>[2x]LECHNQQSSQTPTTTGCSGGETNCYKKRWRD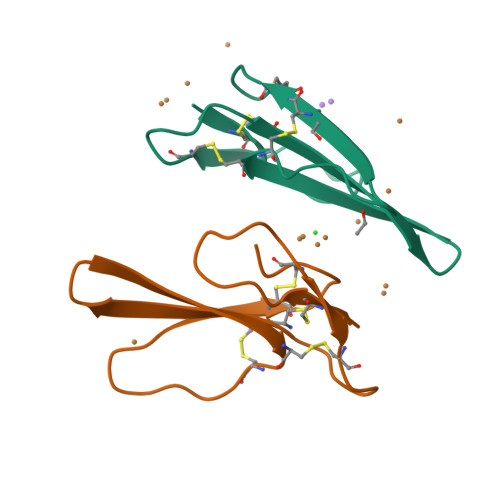HRGYRTERGCGCPSVKNGIEINCCTTDRCNN>[2x]GPGSEFDPGLPSTEDVILKTEQVTKNIQELLRAAQEFKHDSFVPCSEKIHLAVTEMASLFPKRPALEPVRSSLRLLNASAYRLQSECRKTVPPEPGAPVDFQLLTQQV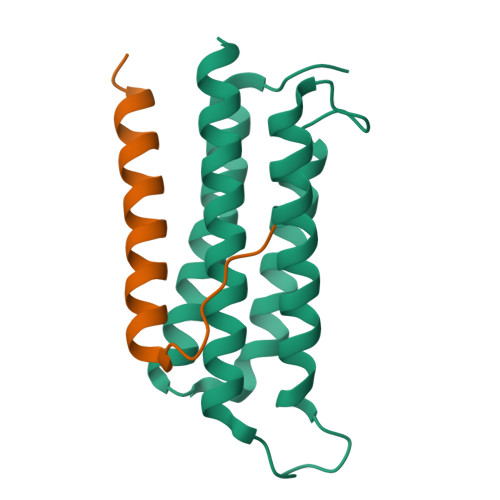IQCAYDIAKAAKQLVTITTREKKQ;>GPGSEFGHSDAQTLAMMLQEQLDAINKEIRLIQEEK[2x]We have been exploring the use of Cry3Aa protein crystals produced in Bacillus thuringiensis (Bt) for multiple applications. The unique biological self-assembly properties of the Cry3Aa protein enable the direct immobilization of functional proteins by genetic fusion or the entrapment of co-expressed protein targets within the Cry3Aa lattice in a fashion that stabilizes the immobilized protein against thermal and solvent denaturation. Here, we report the generation of mechano-responsive PEI-modified Cry3Aa protein crystals and their use for NADH recycling over multiple reaction cycles. We have developed a mechanoresponsive polyethylenimine-modified Cry3Aa (PEI-3A) crystal that enables the versatile and long-term recycling of NADH in an approach that is simple to operate.

Given that the more positively charged Pos3Aa crystals bound NADH better than Cry3Aa crystals (11.2 ± 0.7 and 6 ± 2 μmol/g, respectively), we decided to explore the use of protein cationization to improve NADH binding by incorporating the highly positively charged and flexible PEI polymer into the crystal. PEI-3A crystals were produced by incubating Cry3Aa crystals with PEI in the presence of EDC/NHS. To elucidate the impact of PEI-cationization on the structure of the Cry3Aa crystals, we took advantage of the fact that in vitro-produced Cry3Aa crystals have the same space group and unit cell as the crystals produced in Bt. SEM and X-ray crystallographic analyses of the in vitro-grown Cry3Aa crystals revealed that the crystal framework was unaffected by PEI-modification. The crystal structure also gave no evidence of an ordered PEI monomer or specific residue for PEI attachment, suggesting that, while the PEI molecules bind to the Asp and Glu residues within the nanochannels of the crystal, they are anchored randomly. Similar to what was observed with the Cry3Aa crystals produced in vivo, confocal microscopy confirmed the labeling of PEI and binding of NADH throughout the in vitro-grown PEI-Cry3Aa crystals. Analysis of the size distribution of soluble PEI polymers remaining after the PEI-labeling reaction of Cry3Aa crystals suggests that the 5 nm diameter nanochannels of Cry3Aa (inset) favor PEI polymers smaller than this size. As expected, while the original Cry3Aa crystals had a zeta potential of −35 mV, PEI-modification led to a change to +45 mV. Notably, PEI-cationization of Cry3Aa crystals was highly effective in promoting high levels of NADH binding (540 ± 6 μmol/g) —an amount that we hypothesized should be sufficient for facilitating NADH-dependent enzyme reactions. We speculate that the nanochannels of the Cry3Aa crystals and the nature of the interior of the channel provide an optimal environment for the binding of PEI and, subsequently, NADH.

> MNPNNRSEHDTIKTTENNEVPTNHVQYPLAETPNPTLEDLNYKEFLRMTADNNTEALDSSTTKDVIQKGISVVGDLLGVVGFPFGGALVSFYTNFLNTIWPSEDPWKAFMEQVEALMDQKIADYAKNKALAELQGLQNNVEDYVSALSSWQKNPVSSRNPHSQGRIRELFSQAESHFRNSMPSFAISGYEVLFLTTYAQAANTHLFLLKDAQIYGEEWGYEKEDIAEFYKRQLKLTQEYTDHCVKWYNVGLDKLRGSSYESWVNFNRYRREMTLTVLDLIALFPLYDVRLYPKEVKTELTRDVLTDPIVGVNNLRGYGTTFSNIENYIRKPHLFDYLHRIQFHTRFQPGYYGNDSFNYWSGNYVSTRPSIGSNDIITSPFYGNKSSEPVQNLEFNGEKVYRAVANTNLAVWPSAVYSGVTKVEFSQYNDQTDEASTQTYDSKRNVGAVSWDSIDQLPPETTDEPLEKGYSHQLNYVMCFLMQGSRGTIPVLTWTHKSVDFFNMIDSKKITQLPLVKAYKLQSGASVVAGPRFTGGDIIQCTENGSAATIYVTPDVSYSQKYRARIHYASTSQITFTLSLDGAPFNQYYFDKTINKGDTLTYNSFNLASFSTPFELSGNNLQIGVTGLSAGDKVYIDKIEFIPVN>GPLGSDKALKMPASRYLTDMTLEEMSRDWFMLMPKQKVAGSLCIKMDQAIMDKTIILKANFSVIFDRLETLILLRAFTEEGAIVGEISPLPSLPGHTGEDVKNAIGVLIGGLEWNDNTVRVTETIQRFAWRNS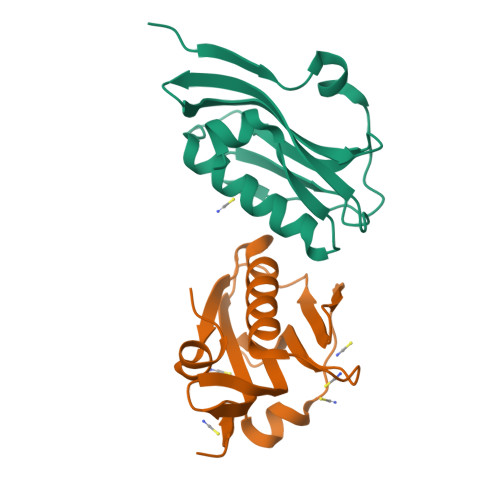DEDGRLPLPPNQKR[4x]Hantaviruses deliver their tripartite genome into the cytoplasm by fusion of the viral and endosomal membranes in response to the reduced pH of the endosome. Here we present the crystal structure of glycoprotein C (GC) from Puumala virus (PUUV), a representative member of the Hantavirus genus. The crystal structure shows GC as the membrane fusion effector of PUUV and it presents a class II membrane fusion protein fold. Furthermore, GC was crystallized in its post-fusion trimeric conformation that until now had been observed only in Flavi- and Togaviridae family members.

Nevertheless, in both PUUV sGc structures, one molecule in the asymmetric unit assembles into a homotrimer around the crystallographic three-fold axis. The protomers adopt the post-fusion domain arrangement, resembling other class II post-fusion structures. They associate in a parallel arrangement with the fusion loop placed at the same end of a stable elongated molecule. The last residue visible in both of our structures is T1076, which lays ~30 Å from the fusion loop. The most notable one is at the membrane proximal part of domain II, close to the fusion loop, where E770 forms a salt-bridge with R902 from the neighboring molecule, thereby stabilizing the trimer in the membrane-proximal region. In our crystal structure we observed N-linked glycans only on N937 whereas N898 is buried in the trimer interface with no available space to accommodate a glycan chain. In contrast to other class II post-fusion trimers, where the glycans decorate the perimeter of the trimer assembly, in PUUV GC the glycans linked to N937 are tightly packed between domain II of one protomer and domain III of the neighboring protomer. Interestingly, R1074 side chain at the N-terminal of the stem is inserted into a negatively charged cavity at the same protomer. The main-chain carbonyls of G883, D884, K893 and C894 create the cavity’s negative charge and lead the stem to a canyon formed by two adjacent protomers. Triangles area for pH 6.0 and pH 8.0 are 52.4 Å2 and 114.1 Å2, respectively. We did not observe any significant differences in rotamers of histidine residues between the low and high pH crystal form.

> ETQNLNAGWTDTAHGSGIIPMKTDLELDFSLPSSASYTYRRQLQNPANEQEKIPFHLQLSKQVIHAEIQHLGHWMDATFNLKTAFHCYGSCEKYAYPWQTAGCFIEKDYEYETGWGCNPPDCPGVGTGCTACGVYLDKLKSVGKVFKIVSLRYTRKVCIQLGTEQTCKTVDSNDCLITTSVKVCLIGTISKFQPSDTLLFLGPLQQGGLIFKQWCTTTCQFGDPGDIMSTPTGMKCPELNGSFRKKCAFATTPVCQFDGNTISGYKRMIATKDSFQSFNVTEPHISTSALEWIDPDSSLRDHINVIVSRDLSFQDLSETPCQIDLATASIDGAWGSGVGFNLVCTVSLTECSAFLTSIKACDAAMCYGSTTANLVRGQNTIHIVGKGGHSGSKFMCCHDTKCSSTGLVAAAPHLDRVTGYNQADSDKIFDDGAPECGMSCWFKKSGEW> RVLYVGNLDKAITEDI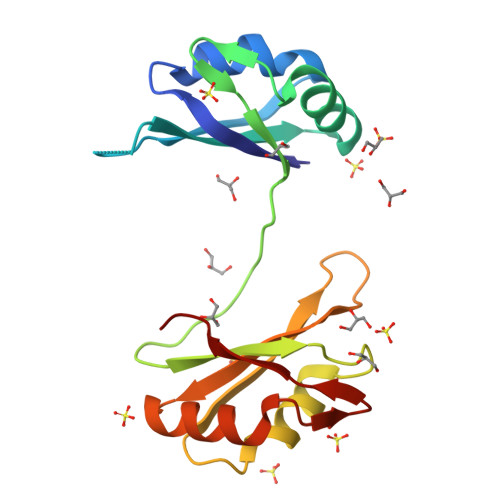LKQYFQVGGPIANIKIMIDKNNKNVNYAFVEYHQSHDANIALQTLNGKQIENNIVKINWAFQSQQSSSDDTFNLFVGDLNVNVDDETLRNAFKDFPSYLSGHVMWDMQTGSSRGYGFVSFTSQDDAQNAMDSMQGQDLNGRPLRINWAAK>HLGPQFCKSCWFENKGLVECNNHYLCLNCLTLLLSVS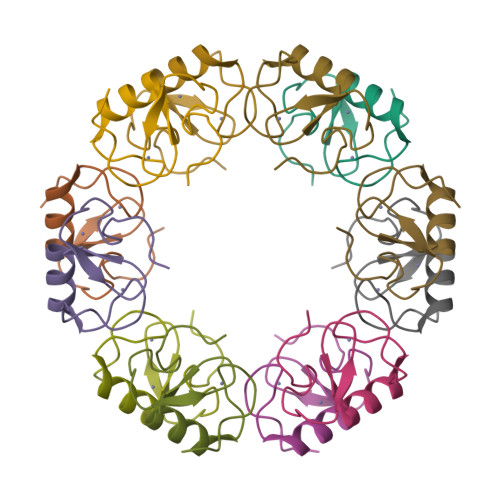NRCPICKMPLPTKLRP[2x]> HGDNNSKPKPGGNSGNRGNNGDGASAKVGEITITPDNSKPGRYISSNPEYSLLAKLIDAESIKGTEVYTFHTRKGQYVKVTVPDSNIDKMRVDYVNWKGPKYNNKLVKRFVSQFLLFRKEEKEKNEKEALLKASELVSGMGDKLGEYLGVKYKNVAKEVANDIKNFHGRNIRSYNEAMASLNKVLANPKMKVNKSDKDAIVNAWKQVNAKDMANKIGNLGKAFKVADLAIKVEKIREKSIEGYNTGNWGPLLLEVESWIIGGVVAGVAISLFGAVLSFLPISGLAVTALGVIGIMTISYLSSFID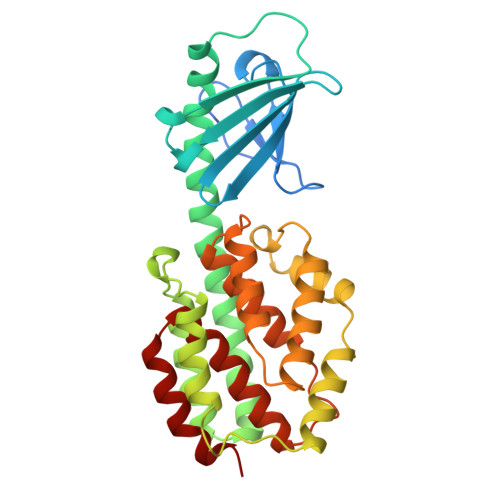ANRVSNINNIISSVIR> MSLPLRHALENVTSVDRILEDLLVRFIINCPNEDLSSVERELFHFEEASWFYTDFIKLMNPTLPSLKIKSFAQLIIKLCPLVWKWDIRVDEALQQFSKYKKSIPVRGAAIFNENLSKILLVQGT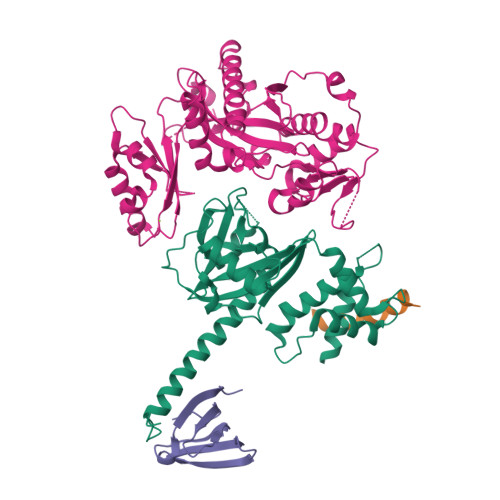ESDSWSFPRGKISKDENDIDCCIREVKEEIGFDLTDYIDDNQFIERNIQGKNYKIFLISGVSEVFNFKPQVRNEIDKIEWFDFKKISKTMYKSNIKYYLINSMMRPLSMWLRHQRQIKNEDQLKSYAEEQLKLLLGITKEEQIDPGRHHHHHH;> GPLGSMTGAATAAENSATQLEFYRKALNFNVIGRYDPKIKQLLFHTPHASLYKWDFKKDEWNKLEYQGVLAIYLRDVSQNTNLLPVSPQEVDIFDSQNGSNNIQVNNGSDNSNRNSSGNGNSYKSNDSLTYNCGKTLSGKDIYNYGLIILNRINPDNFSMGIVPNSVVNKRKVFNAEEDTLNPLECMGVEVKDELVIIKNLKHEVYGIWIHTVSDRQNIYELIKYLLENEPKDSFA;> GPLGSMSQFVGFGVQVELKDGKLIQGKIAKATSKGLTLNDVQFGDGGKSQAFKVRASRLKDLKVLTVASQS;> GPLGSSKTNNLIVVSIDPMEYIYKPLTHALKKYLPQVEIVSNLPEFDNGGCEKEMKVFHYGDYEQLDMDKLMELPNNYFTNSYIYRKALIRKHFLSHTIQTYTAKNPESILKKAYLESFTIDLDYAEFLDDALDENWELRQELENESQDKWWIVKPSMSDKGQGIRVFKTIEDLQAIFDSFDDEDSEAEESGNDDDADDVNGEFMDNNKVNISQLRHFIIQEYLTNPLLLASMDNRKFHIRCYVVCRGDLQVFVYDRMLALFAAKPFVPLDPYAYSVTDLKDLECHLTNTCLQSKKKDKDSSVLEFDSIEEIPNERKSNIKEQIHSITNDVFLAAVNVNRLNFQPLPNAFETYGVDFLIDSNYEVKLLEINAFPDFKQTGKDLKNLIDELFDDTVKYCVTPIFNENRNKTDDETDPNFVKVIDYTSNGW>[8x]GHMSAPIKANDPNGEV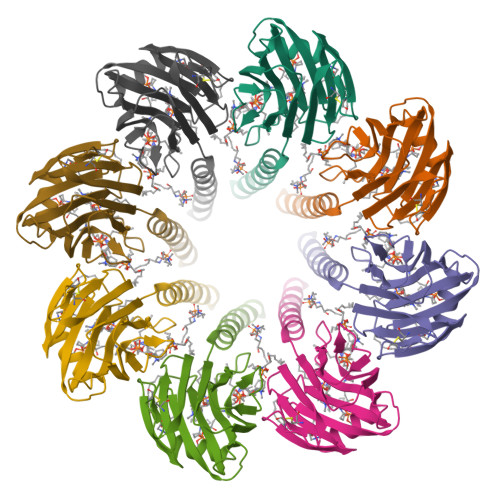LEEMPKTKRGAEALLADVGLAHFPEMVPNRQELRALLKRSHNAEAIPQEPMDLENLDSEKRAARIAAGTIIAGAELTIGLLQNLLDVLANVNRKCAVGVDNESGFRWQEGSTYFFSGTADENLPYSVSDGYAVLYGPRKTNGPVATGVVGVLAYYIPSIGKTLAVMWSVPFDYNFYQNWWNAKLYSGNQDADYDHYVDLYYDANPFKANGWHERSLGSGLKFCGSMSSSGQATLEIHVLKESETCM>MPPETATNPKDARHDGWQTLKRFLPYLWPADNAVLRRRVVGAILMVLLGKATTLALPFAYKKAVDAMTLGGGAQPALTVALAFVLAYALGRFSGVLFDNLRNIVFERVGQDATRHLAENVFARLHKLSLRFHLARRTGEVTKVIERGTKSIDTMLYFLLFNIAPTVIELTAVIVIFWLNFGLGLVTATILAVIAYVWTTRTITEWRTHLREKMNRLDGQALARAVDSLLNYETVKYFGAESREEARYASAARAYADAAVKSENSLGLLNIAQALIVNLLMAGAMAWTVYGWSQGKLTVGDLVFVNTYLTQLFRPLDMLGMVYRTIRQGLIDMAEMFRLIDTHIEVADVPNAPALVVNRPSVTFDNVVFGYDRDREILHGLSFEVAAGSRVAIVGPSGAGKSTIARLLFRFYDPWEGRILIDGQDIAHVTQTSLRAALGIVPQDSVLFNDTIGYNIAYGRDGASRAEVDAAAKGAAIADFIARLPQGYDTEVGERGLKLSGGEKQRVAIARTLVKNPPILLFDEATSALDTRTEQDILS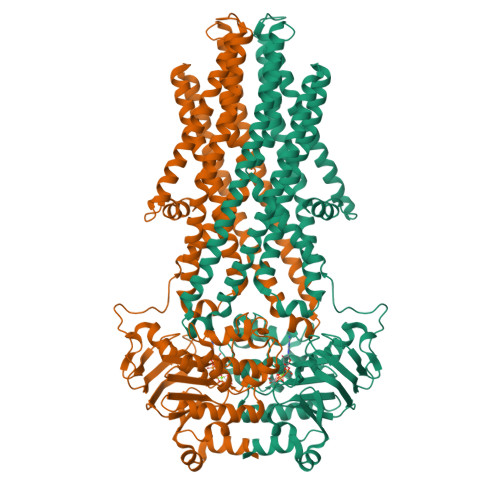TMRAVASHRTTISIAHRLSTIADSDTILVLDQGRLAEQGSHLDLLRRDGLYAEMWARQAAESAEVSEAAEHHHHHH[2x]> SPHVFISYSWSSEDHKEWVLDLANKLMKESGVEVILDRWHGVV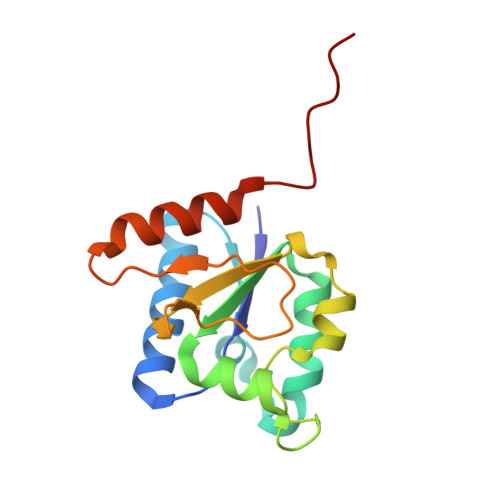GHDRFEFMENSIKIADKVLVICDKDYCEKANTRRGGVGTETMIITPNIYNNTKQEKFIPISLGEENGEYFLPDFFKSRFALGWNYEDIDKSYKELERLIWEEPLLKPPVRG> MLRISQEALTFDDVLLIPGYSEVLPKDVSLKTRLTRGIELNIPLVSAAMDTVTEARLAIAMAQEGGIGIIHKNMGIEQQAAEVRKVKKHETAIVRDPVTVTPSTKIIELLQMAREYGFSGFPVVEQGELVGIVTGRDLRVKPNAGDTVAAIMTPKDKLVTAREGTPLEEMKAKLYENRIEKMLVVDENFYLRGLVTFRNIEKAKTYPLASKDEQGRLRVGAAVGTGADTG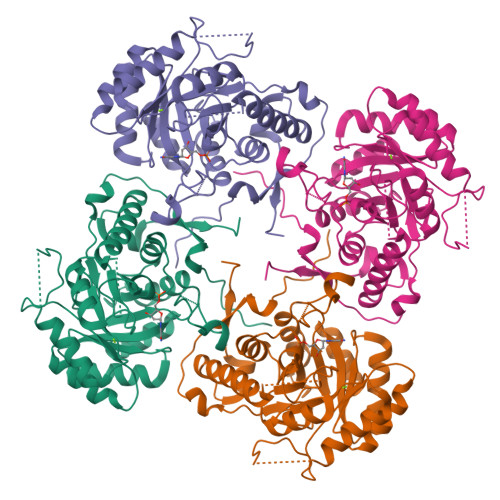ERVAALVAAGVDVVVVDTAHGHSKGVIERVRWVKQTFPDVQVIGGNIATAEAAKALAEAGADAVKVGIGPGSICTTRIVAGVGVPQISAIANVAAALEGTGVPLIADGGIRFSGDLAKAMVAGAYCVMMGSMFAGTEEAPGEIELFQGRSYKSYRGMGSLGAMSGSQGSSDRYFQDASAGAEKLVPEGIEGRVPYKGALSAIVHQLMGGLRAAMGYTGSADIQQMRTQPQFVRITGAGMAESHVHDVQITKEAPNYRVG> MKSLKGSRTEKNILTAFAGESQARNRYNYFGGQAKKDGFVQISDIFAETADQEREHAKRLFKFLEGGDLEIVAAFPAGIIADTHANLIASAAGEHHEYTEMYPSFARIAREEGYEEIARVFASIAVAEEFH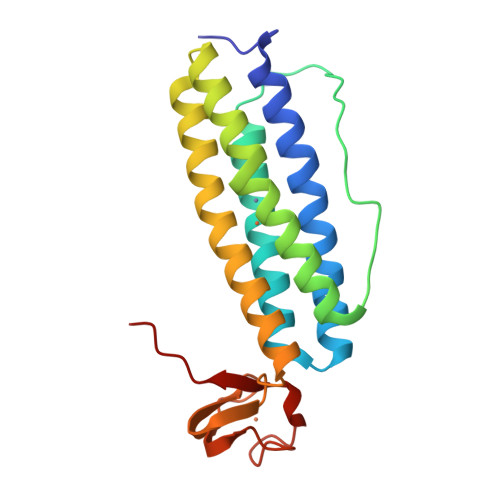EKRFLDFARNIKEGRVFLREQATKWRCRNCGYVHEGTGAPELCPACAHPKAHFELLGINW> GPSKIEEVKSTTKTQRIASHSHVKGLGLDESGLAKQAASGLVGQENAREACGVIVELIKSKKMAGRAVLLAGPPGTGKTALALAIAQELGSKVPFCPMVGSEVYSTEIKKTEVLMENFRRAIGLRIKEGPPGIIQDVTLHDLDVANARPQGGQDILSMMGQLMKPKKTEITDKLRGEINKVVNKYIDQGIAELVPGVLFVDEVHMLDIECFTYLHRALESSIAPIVIFASNRGNCVIRGTEDITSPHGIPLDLLDRVMIIRTMLYTPQEMKQIIKIRAQTEGINISEEALNHLGEIGTKTTLRYSVQLLTPANLLAKINGKDSIEKEHVEEISELFYDAKSSAKILA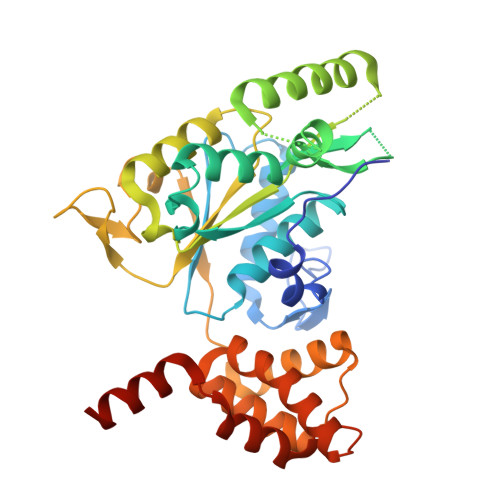DQQDKYMK>MGRIKNKQFAVIGLGRFGGSICKELHRMGHEVLAVDINEEKVNAYASYATHAVIANATEENELLSLGIRNF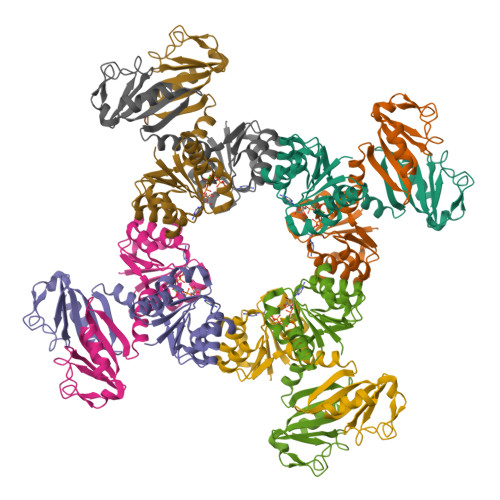EYVIVAIGANIQASTLTTLLLKELDIPNIWVKAQNYYHHKVLEKIGADRIIHPEKDMGVKIAQSLSDENVLNYIDLSDEYSIVELLATRKLDSKSIIDLNVRAKYGCTILAIKHHGDICLSPAPEDIIREQDCLVIMGHKKDIKRFENEGM[2x]>[2x]GMERILKKQPAP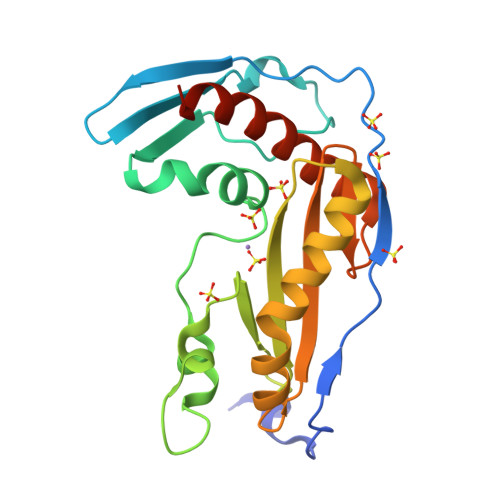VRALTIHPLRRYESSIYDTPIPAYVIKHSSDGVTIDIATSELADGQSGSTIQPFESVPAQNLTLFKHDFTFGHLADTTDKKFVEVFGVLENRADDSDFQSPDMIIETETGHVYVVEFTTTMGDANSADLAARNKIAKYEIACLDRSAIKPISLYIIAVHFNGVVSNLDLSDEEVNEIVFRFRLARDIFEELREINPALFD> PRGGGSAGAPNGCTNNPKHPPG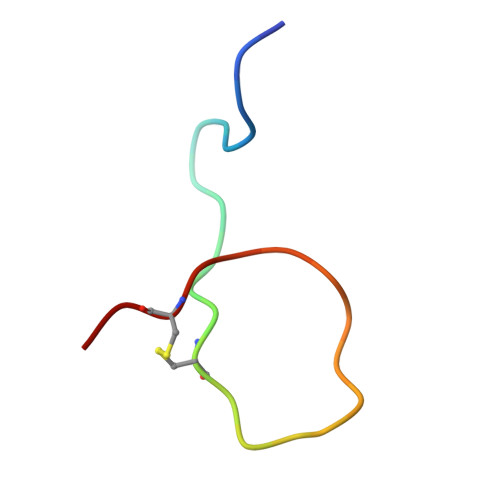GKCHG>[4x]MNCDNAKFIIFFFFIIFLCANFAVCNELEDYVEKSVNSETKLHKLADFAIDWAHNNGLILRTKQFLNKSDVAEFAPVSLLPSPFPRHAFEKAVAV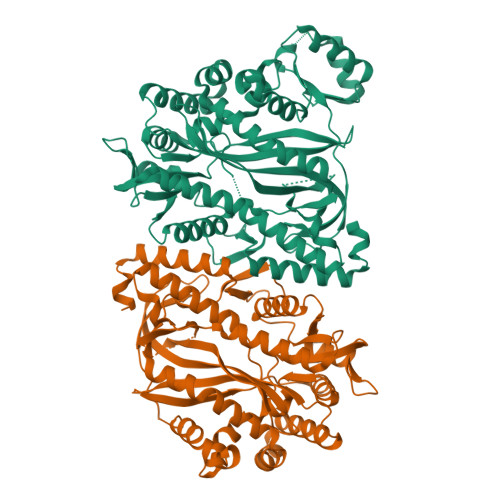HEALQLLYFRVACDYEFMMDAYKDVVNTDNHLRQLVNIIKDAHKQGIKQPTTLLIMRADYMLNTLNSKGNDDEYELKQVEVNTGAIGGLGIDRRTTELHRQMLRKVGMDTSNSPANNGDSNMIESLFMAWEAFGNKNALFVFLSHERLQYKFELRNIQCQLEELSNGQMKVEYVSLKAGYEQLKLGEDYSLLLNGEIVGVVYSTISALGHQANAREMEARRTIELSNAIKAPSLAIAISSSKKIQQLLTTPGTLERFFPSATEADKVAAIRETFTGLWGLEKSDDQTERRIKDAIENPANYVLKSNGECGGNNFYDEALAEKLRTMPQAERASHILMQKLIPMATKNYFLRPFHEPKLNVVVGELGVNGTLLGNLRDQSVRHNVQSGHLLRTKLREANEGGISVGTGVGDSPYLF In bacteria, expression of folate-related genes is controlled by the tetrahydrofolate (THF) riboswitch in response to specific binding of THF and its derivatives. Recently, a second class of THF riboswitches, named THF-II, was identified in Gram-negative bacteria, which exhibit distinct architecture from the previously characterized THF-I riboswitches found in Gram-positive bacteria. Distinct from the aptamers of the previous THF-I riboswitch found in Gram-positive bacteria, the THF-II riboswitch aptamer adopts a simple architecture in which the secondary structure consists of two helices of P1 and P2, two junctions of J12 and J21, and an apical loop L2. The RNA in the ligand–RNA complexes adopts a long rod-like, continuously stacked helix structure stabilized by two helices of P1 and P2 and the interconnecting ligand-bound binding pocket.

Our ITC experiments indicated that the C22G mutant lost the binding activity to THF. We then determined the crystal structure of the C22G mutant of THF-II-lotiTL RNA (THF-II-lotiTL-C22G), which diffracted to 3.22 Å. The space group of the crystal is P3121, in which one asymmetry unit contains only one RNA molecule. The overall crystal structure of THF-II-lotiTL-C22G is highly similar to that of WT RNA, between which the RMSD is 0.7 Å. The structural differences mainly lie in the J12 junction loop. In the C22G mutant, U18 intercalates into the binding pocket and forms a Hoogsteen base pair with A21. In contrast, U18 in WT RNA is flipped out of the binding pocket and stacked with C19. Furthermore, the N2 of G22 forms one hydrogen bond with O2 (carbonyl) of U44, mimicking the ligand-bound conformation in WT RNA. Interestingly, a hydrogen bond is formed between O2' (hydroxyl) of U18 and OP2 of A21, which may position the O2' (hydroxyl) of U18 in an in-line position, thus explaining a previous observation from in-line probing that the C to G mutation results in a similarly robust cleavage product at U18 to WT RNA. The ligand unresponsiveness and reduced RBS accessibility are understandable since the C22G mutant loses the ligand-binding activity and can be a mimic of the ligand-bound THF-II riboswitch.

> GGCGUGGUCCGUUCAAGUCGUUCCUCGAAAGAGGAACUACGGGAGACGCC ethyl 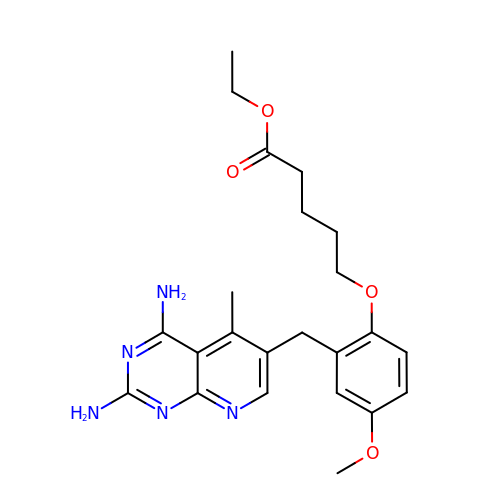5-{2-[(2,4-diamino-5-methylpyrido[2,3-d]pyrimidin-6-yl)methyl]-4-methoxyphenoxy}pentanoate | C23 H29 N5 O4 | BHQORMWWDFDSIW-UHFFFAOYSA-N> MGVIKKKRSHHGKASRQQYYSGVQVGGVGSMGAINNNIPSLTSFAEENNYQYGYSGSSAGMNGRSLTYAQQQLNKQRQDFERVRLRPEQLSNIIHDESDTISFRSNLLKNFISSNDAFNMLSLTTVPCDRIEKSRLFSEKTIRYLMQK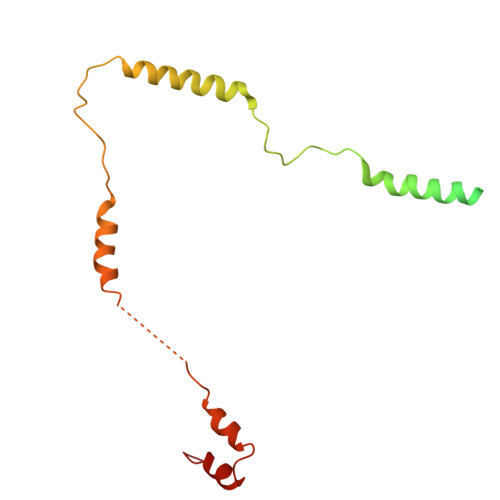QHXXXXXXXXXXXXXXXXXXXXXXXXXXXXX>GRRKRTAVTGSQTALLLRAFE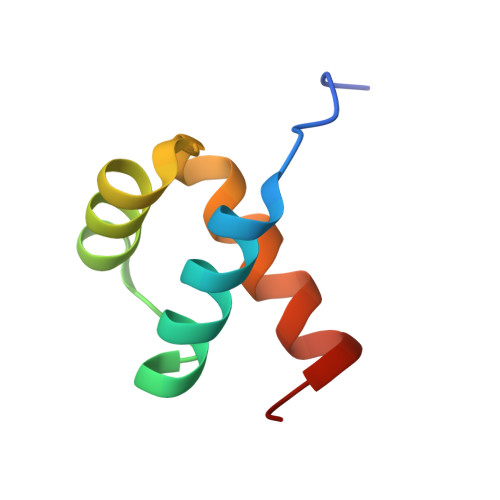KDRFPGIAAREELARETGLPESRIQIWFQNRRARHPGQG[2x]Mycobacterium tuberculosis DNA gyrase, an indispensable nanomachine involved in the regulation of DNA topology, is the only type II topoisomerase present in this organism and is hence the sole target for quinolone action, a crucial drug active against multidrug-resistant tuberculosis. DNA gyrase and topoisomerase IV consist of two subunits (GyrA and GyrB in DNA gyrase, ParC and ParE in topoisomerase IV), which form the catalytically active heterotetrameric complex (i.e. A2B2 and C2E2, respectively). The GyrB Toprim and GyrA breakage-reunion domains come from separate subunits and cooperatively form the enzyme core. The breakage-reunion domain contains the catalytic tyrosine responsible for the cleavage and religation of the DNA double helix.

We solved two high resolution structures of the Toprim domain displaying two different conformations of the metal-binding site, to 2.1 and 1.95 Å resolution, respectively. TopBK was crystallized in presence of magnesium (crystal I) and calcium (crystal II) and the structures were solved at 2.1 Å and 1.95 Å resolution, respectively, with one monomer in the asymmetric unit in both cases. When magnesium is substituted in the crystallization conditions by calcium (TopBK crystal II), side chains of the triad are observed in an inactive conformation similar to the one observed for the low resolution M. tuberculosis Toprim domain structure. The structure displays a two-domain organization, a globular domain constituted by discontinuous segments (residues 448–564 and 633–654) and the Tail domain (residues 565–608) connected by a loop-helix-loop hinge region (residues 609–632). In the globular domain, the conserved acidic triad (E459, D532, D534), which constitutes the signature of the Toprim domain, binds the magnesium ion essential for the catalysis of the cleavage-ligation reaction. The Toprim domain forms a dimer with a symmetry related molecule in both crystal structures (crystal I and II), burying 1017 Å2 at the protein-protein interface, indicative of a biologically relevant interaction. Surprisingly, the high resolution structures of TopBK, revealed two disordered regions, between β1 and β2 (residues 460–474) and between β2 and α2 (residues 484–492). These regions are structured in the context of the catalytic core or in presence of DNA. The second disordered region, the loop between β2 and α2, is exposed to the solvent explaining its high flexibility. In the structures of type II topoisomerases in complex with DNA, this loop (hereafter named DBL for DNA-Binding Loop) constitutes the interface between the Toprim domain and DNA and is stabilized through protein-DNA interactions.

> MAHHHHHHVDDDDKTDPRKSELYVVEGDSAGGSAKSGRDSMFQAILPLRGKIINVEKARIDRVLKNTEVQAIITALGTGIHDEFDIGKLRYHKIVLMADADVDGQHISTLLLTLLFRFMRPLIENGHVFLAQPPLYKLKWQRSDPEFAYSDRERDGLLEAGLKAGKKINKEDGIQRYKGLGEMDAKELWETTMDPSVRVLRQVTLDDAAAADELFSILMGEDVDARRSFITRNAKDVRFLDV> GSGFTSKDTYLSHFNPRDYLEKYYKFGSRHSAESQILKHLLKNLFKIFCLDGVKGDLLIDIGSGPTIYQLLSACESFKEIVVTDYSDQNLQELEKWLKKEPAAFDWSPVVTYVCDLEGNRVKGPEKEEKLRQAVKQVLKCDVTQSQPLGAVPLPPADCVLSTLCLDAACPDLPTYCRAL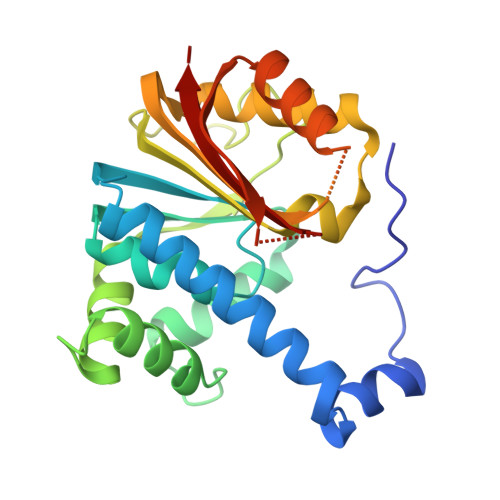RNLGSLLKPGGFLVIMDALKSSYYMIGEQKFSSLPLGREAVEAAVKEAGYTIEWFEVISQSYSSTMANNEGLFSLVARKL> MFENDILVAGGDPGFGAIKLDAGDTKVLFPAVICKGNERIFSALGNGNVSRGTDEEMQTGSLDVIVTNHSTGVSRHYFMGSLAESLNPNEAHYCWDEDKSTDEEATALLVVALAVAQKEPKANIYLGTGVPVKYYAALKDKYEAELKGTWSVAFRSGPFKGQTRQLTIIRSRVLPQSYGVFIKETLNEYGIPISPKLFNGYVVVIDPGFRTTDVATFYDGVMLDPPNSFSIEKGLKWAYTGVAEQLKEMTINHANPIETDDKELDKVFRVNEGMYPWNNGAINLNPVMQDMLGQLGTDISREVKKSLKPMLGKIHTVLVAGKVGEMIFEHLQFENKVLIENPQFGNATGFRIMAANLVNNITKKANAAP

ParMs generally exist on low-copy number plasmids where they contribute to plasmid segregation and stable inheritance. Here we report the discovery and characterization of two chromosome-encoded ParMs (cParMs) from the genomes of Desulfitobacterium hafniense (Dh-cParM1) and Clostridium botulinum (Cb-cParM). Both cParMs form filaments, exhibit nucleotide hydrolysis, and possess characteristic ParM subunit structures.

Dh-cParM1 forms single and tightly coupled double filaments and is highly conserved on the chromosomes of five of six Desulfitobacterium species. From a total of 2845 images and a final selection of 71,060 particles, a 4.0 Å resolution density map of a Dh-cParM1 single filament constructed from two parallel strands was reconstructed displaying a helical rise and twist of 24.5 Å and 156.03°, respectively. Its short helical repeat is about half that of F-actin or ParM-R1 resulting in a more twisted structure. The single filament structure is constructed from two parallel, staggered protofilaments. As observed for other ParM protomers, the analogous subdomain 2 region to the DNase I binding loop in actin was clearly observed in the density as well as the characteristic ParM closed beta-barrel in subdomain 1. Due to the limited resolution, we cannot unambiguously determine the state of the nucleotide bound in this structure. However, ADP appears to fit better into the cryoEM density map than ATP, which is consistent with polymerization initiating hydrolysis of ATP. The interacting residues surrounding the nucleotide bear similarity to those of ParM-R1. The hydrophobic residues of subdomain 2 interact with the hydrophobic pocket of subdomains 1 and 3 of the upper subunits in a ball and socket manner, similar to that observed in pCBH ParM. The maps from class 2 with GTP (30 min) and the third condition (GTP, 1 min) were similar to each other, although the resolution was limited, suggesting that they were in the state before the phosphate release. The helical twists for Cb-cParM and Dh-cParM1 protofilaments were different, ∼167° compared to ∼156°, respectively, with Cb-cParM being more similar to ParM-R1 (∼165°).> MTSLYAPGAEDIRQRLRPFGFFFEKSLKDLIKGIRSHNETPEKLDQFFKQVLSECREEVNSPDLNSKTNAVLKLTYLEMYGFDMAWCNFHILEVMSSNKLQQKRVGYLAASQSFYKDSDILMLATNLLKKDLKYDGNNDVVKVGIALSGLSTIITPSLARDIADDLFTMLNSTRPYIRKKAITALFKVFLQYPEALRDNFDKFVSKLDDDDISVVSAAVSVICELSKKNPQPFIQLSPLLYEILVTIDNNWIIIRLLKLFTNLSQVEPKLRAKLLPKILELMESTVATSVIYESVNCIVKGNMLEEDDFETAMACLERLHTFCDSQDPNLRYISCILFYKIGKINTDFISRFDQLIIRLLSDVDVSIRSKAIELVEGIVDEDNLKAIVQTLMKQFVDEDVVILQTGSIVYEKSKRIPIIIPENYKIKMVNVIISICSADNYSSVNDFEWYNAVIMDLAMLCQDISDKSLGSKIGEQFRNLMIKVPSMREVTIANIIKLISNDNINKQLPTVLRECIWCLGEFSTLVENGNDLIKIMTENISYYSHSVQEVLILALVKVFSNWCNNFQEDKRFEIKMVLKELIEFFENLSYSSTFEVQERSVEVLEFLRLSLEALEEDTEGLPMLLSEVLPSFFNAYELAPIARGTQLKLAVDENLDLETPFLTKEAADELLD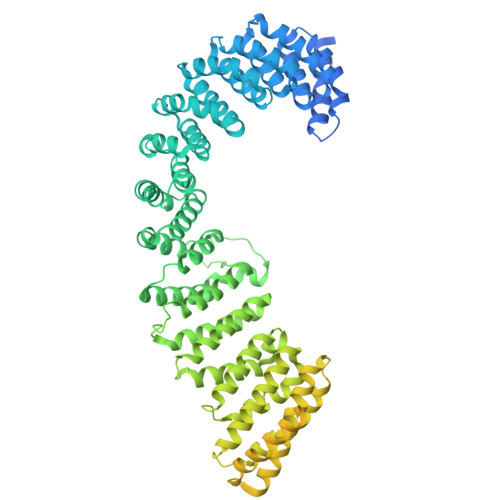EQKSDAISDLMSDISMDEQVELKFVDDSDTSYEEKEKLDDFENPFEIEREKERMSNPYYLGEEDEERTKNSKDLLDLNEEESSDKKPETIRLNRTDNSLNSLSLSTTEISRKKKKGKKKNRVQVLSDEPVIEAAPKRKDAFQKPHDNHSTQNPLKKDKINLRMHSQLENFDFSNFGQSSNAGRGSQEEGNLRKEDELELSRLEANLIVKDEKDNLSDTEEVIVIKKKKKGKKSKSKNKLKTKAKNSPEPNEFLRDQSTDIRTLQVDGSDYKDDDDKDYKDDDDKDYKDDDDK> KAPSQNAI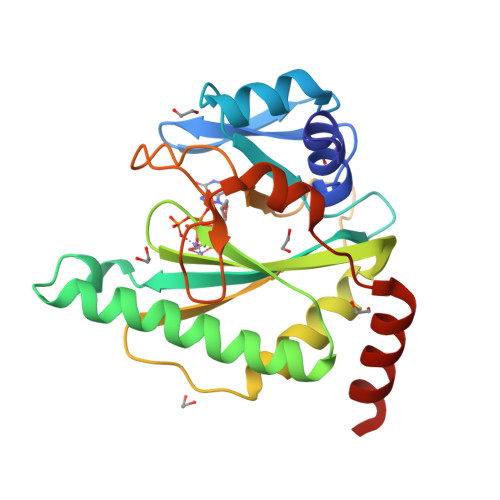KRFMTLFSGREDVFSIQYEGGYRPIRRPLNFQDIKNHFSGKKTLGIYLLKKNDTVKFAAYDIDIKKHYLNREDKFVYEENSKKVAKRLSRELNLENITHYFEFTGNRGYHIWIFFDIPVSAYKIKYIMEKILDRIELEEGIDVEIFPKQTSLNGGLGNLIKVPLGVHKKTGKKCLFVDNDFNVIENQIEFLNNIKENKATEINKLFREIFNEND>[6x]PPGPPGPPG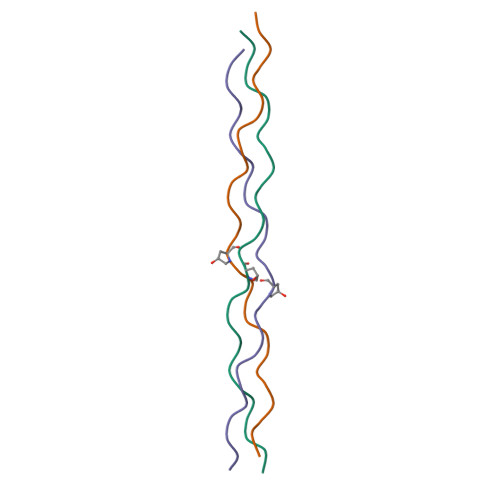PPGPSGPPGPPGPPGPPG> GDHPTFNKITPNLAEFAFSLYRQLAHQSNSTNILFSPVSIAAAFAMLSLGAKGDTHDEILEGLNFNLTEIPEAQIHEGFQELLRTLNQPDSQLQLTTGNGLFLSEGLKLVDKFLEDVKKLYHSEAFTVNFGDTEEAKKQINDYVEKGTQGKIVDLVKELDRDTVFALVNYIFFKGKWERPFEVKDTEEEDFHVDQVTTVKVPMMKRLGMFNIQHSKKLSSWVLLMKYLGNATAIFFLPDEGKLQHLENELTHDIITKFLENEDRRSASLHLPKLSITGTYDLKSVLGQLGITKVFSNGADLSGVTEEAPLKLSK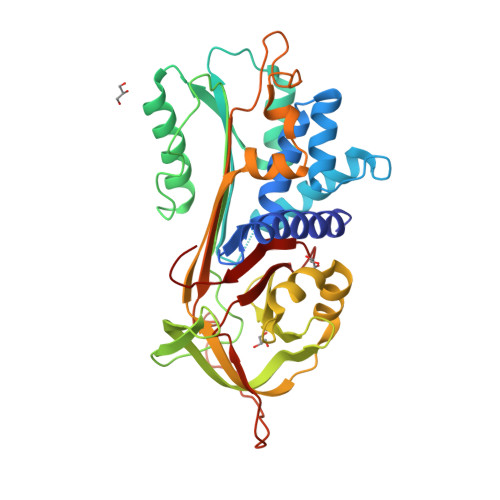AVHKAVLTIDKKGTEAAGAMFLEAIPMSIPPEVKFNKPFVFLIIEQNTKAPLFMGRVVNPTQK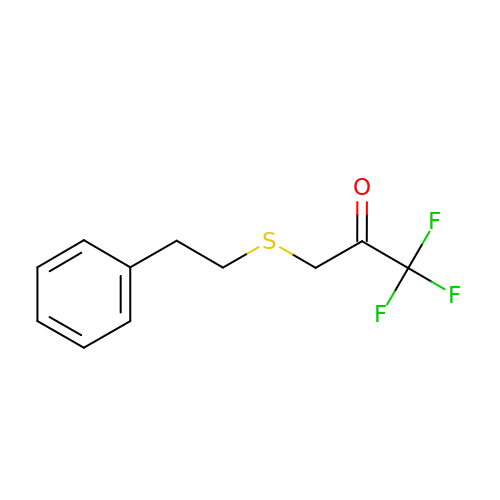1,1,1-trifluoro-3-[(2-phenylethyl)sulfanyl]propan-2-one | C11 H11 F3 O S | UJAGOKUXPHIFEB-UHFFFAOYSA-N> MGEEFEKLMKKFENVNKDGEIVEDEDEWEEFFKQEEYVKIPKDRIAVLIGKKGQTKKEIEKRTKTKITIDSETGEVWITSTKETEDPLAVWKARDIVLAIGRGFSPERAFRLLNEGEYLEIINLTDIIIGNEKNALPRVRGRIIGRKGRTRQIIEEMSGASVSVYGKTVAIIGNPIQIEIAKTAIEKLARGSPHGSVYRYLERRKKDLELEGAMY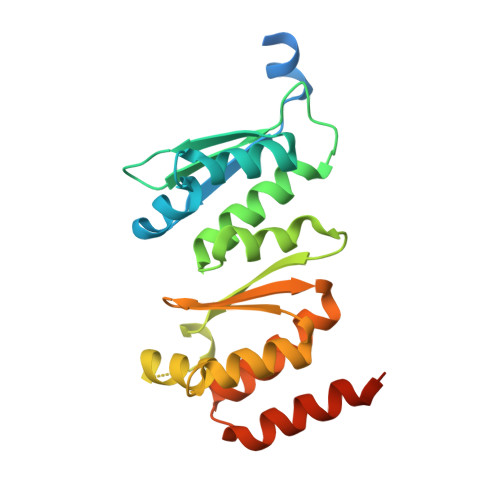YENL> GHMAKTYDYLFKLLLIGDSGVGKSCLLLRFADDTYTESYISTIGVDFKIRTIELDGKTIK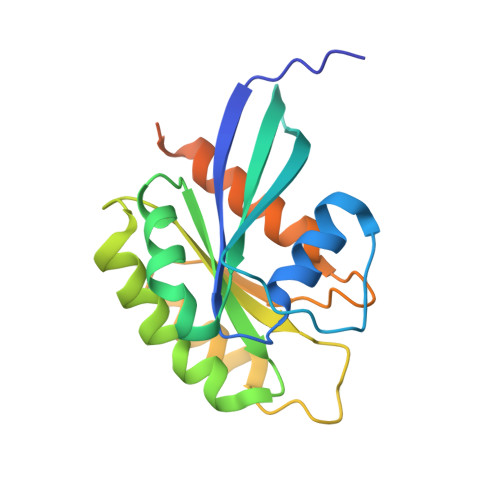LQIWDTAGQERFRTITSSYYRGAHGIIVVYDVTDQESYANVKQWLQEIDRYASENVNKLLVGNKSDLTTKKVVDNTTAKEFADSLGIPFLETSAKNATNVEQAFMTMAAEIKKRMGPGAASGGERPNLKIDSTPVKPAGGGCC> SKSTAEIRQAFLDFFHSKGHQVVASSSLVPHNDPTLLFTNAGMNQFKDVFLGLDKRNYSRATTSQRCVRAGGKHNDLENVGYTARHHTFFEMLGNFSFGDYFKLDAILF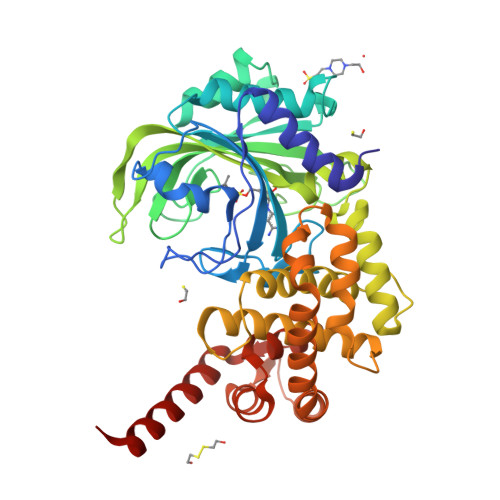AWLLLTSEKWFALPKERLWVTVYESDDEAYEIWEKEVGIPRERIIRIGDNKGAPYASDNFWQMGDTGPCGPCTEIFYDHGDHIWGGPPGSPEEDGDRYIEIWNIVFMQFNRQADGTMEPLPKPSVDTGMGLERIAAVLQHVNSNYDIDLFRTLIQAVAKVTGATDLSNKSLRVIADHIRSCAFLIADGVMPSNENRGYVLRRIIRRAVRHGNMLGAKETFFYKLVGPLIDVMGSAGEDLKRQQAQVEQVLKTEEEQFARTLERGLALLDEELAKLSGDTLDGETAFRLYDTYGFPVDLTADVCRERNIKVDEAGFEAAMEEQRRRAREASGF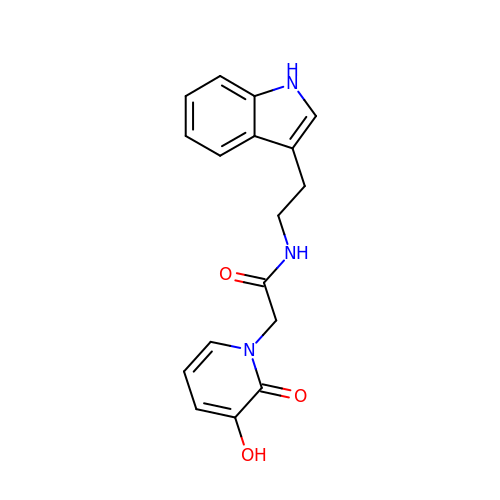~{N}-[2-(1~{H}-indol-3-yl)ethyl]-2-(3-oxidanyl-2-oxidanylidene-pyridin-1-yl)ethanamide | C17 H17 N3 O3 | NRCSONGNAATKNC-UHFFFAOYSA-N>SNATAFVPALVASGLPNEKFCFEGFLPQKKGRQTRLKALAEEHRTMVFYESPHRLLKTLTQFAEYFGTERQATVSREISKLHEETVRGSLAELIEHFTATEPRG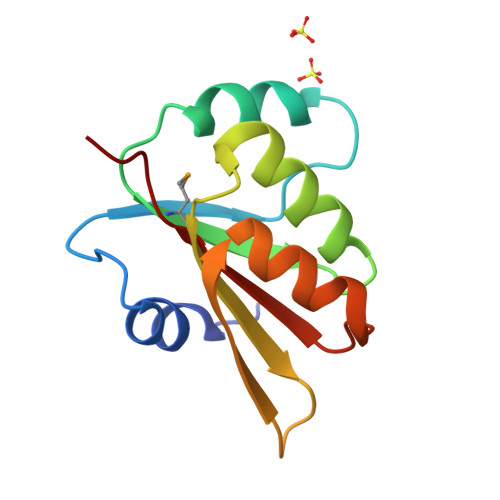EIVIVLAGIDD[2x]Riboswitches are gene regulatory elements that are frequently found in the 5′-untranslated regions of bacterial mRNAs (1–6). Only very recently, the nadA RNA motif has been assigned to function as a riboswitch which regulates the expression of genes involved in biosynthesis of the enzyme cofactor nicotinamide adenine dinucleotide (NAD+). Although the cofactor is ubiquitous, this riboswitch appears to be rather rare and has the special feature of a tandem aptamer architecture. Here, we report crystal structures of the first, as well as the second domain of the NAD+ riboswitch, both individually bound to NAD+.

The non-conserved sequence portion adjoining to stem P1b in domain 1 was dispensable for NAD+ binding as was the non-conserved region adjoining to stem P1b in domain 2. Therefore, they were replaced with GAAA tetra-loops, and in case of domain 1, additionally, with the U1A protein-binding loop in one of the constructs. In co-crystallization with the U1A protein, the crystal structure of the NAD+ riboswitch domain 1 (from Acidobacterium capsulatum ATCC 51196; in the following named 17delU1A-D1/NAD+) was obtained at a resolution of 2.80 Å. The space group was P6122, in which each asymmetric unit contained one molecule. The phase problem of 17delU1A-D1/NAD+ was solved by the SAD method using the anomalous signal of selenium in selenomethionine (Se-Met)-derivatized U1A protein. Therefore, it is not surprising that 17delU1A-D1/NAD+ folds into a similar pseudoknot scaffold as 18GAAA-D1/NAD+, and C12 and C13 from J1 form the characteristic long-distance base-paring interaction with G43 and G45 from J2. In contrast to 18GAAA-D1/NAD+, the 17delU1A-D1/NAD+ dimer involves both junctional regions J1 and J2 in contacts between the individual units. The C11′ from the symmetric molecule forms a Hoogsteen interaction with G45 and hence generates a base triple C11′•G45-C12 that forms an extended stacking interface (with C11•G45′-C12′) between the two molecules in the dimer. Clearly, under the conditions used, both RNAs existed as monomers in solution without any indication for dimer formation.

> ETRPNHTIYINNLNEKIKKDELKKSLHAIFSRFGQILDILVSRSLKMRGQAFVIFKEVSSATNALRSMQGFPFYDKPMRIQYAKTDSDIIAK>GMPKANLEIIRSTYEG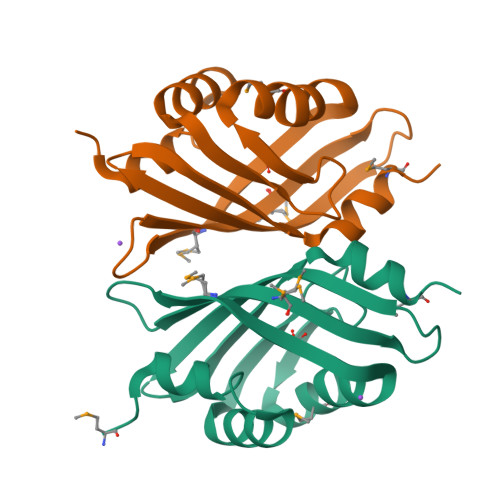SASSNAKHLAEALSEKVEWTEAEGFPYGGTYIGVEAIMENVFSRLGSEWNDYKASVNMYHEVSGKDVIIAEGMYSGVYKDTGKSFEAEFVHVWQLENGKIVKFKQYVDSHLVREAMKS[2x]> KGTDSLKSSIEKYLKDKKAKVGVAVLGIEDNFKLNVNEKHHYPMQSTYKFHLALAVLDKLDKENISIDKKLFVKKSELLPNTWSPLRDKYPDGNVDLSISEILKATVSRSDNNGCDILFRFVGGTNKVHNFISKLGVKNISIKATEEEMHKAWNVQYTNWTTPDATVQLLKKFYKNEILSKNSYDYLLNTMIETTTGPKRLKGLLPDGTVVAHKTGSSDTNDKGITAATNDIGIITLPNGKHFAI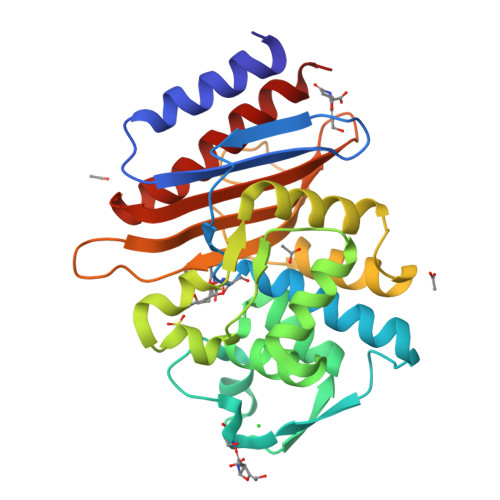AVYVSDSSEKSDVNEKIIAEICKSVWDYLVKD>[3x]MMIRGIRGATTVERDTEEEILQKTKQLLEKIIEENHTKPEDVVQMLLSATPDLHAVFPAKAVRELSGWQYVPVTCMQEMDVTGGLKKCIRVMMTVQTDV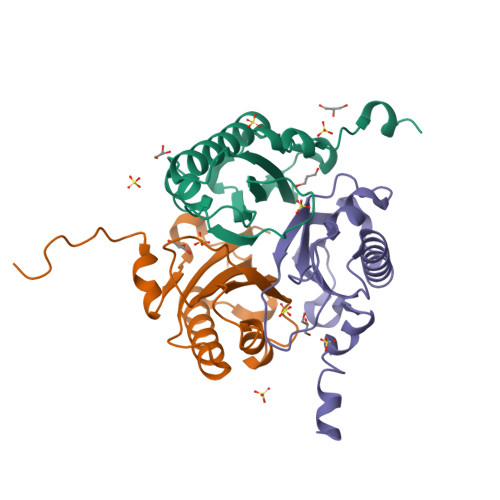PQDQIRHVYLEKAVVLRPDLSLTKNTEL>MHHHHHHDPPCEELEIVWKNIKAEARALADCEPMLASFYHATLLKHENLGSALSYMLANKLASPIMPAIAIREVVEEAYAADPEMIASAACDIQAVRTRDPAVDKYSTPLLYLKGFHALQA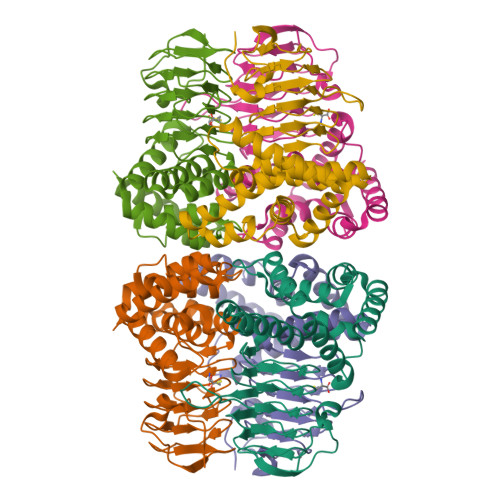YRIGHWLWNKGRRALAIFLQNQVSVSFQVDIHPAAKIGRGIMLDHATGIVVGETAVIEDDVSILQSVTLGGTGKTSGDRHPKIREGVMIGAGAKILGNIEVGRGAKIGAGSVVLQPVPPHTTAAGVPARIVGKPGSDKPSMDMDQHFNGIHHTFEYGDGI[3x]Here, we present the structure of an outer-membrane core complex from the iconic F-T4SS encoded by the E. coli pED208 plasmid solved by single-particle cryo-electron microscopy at 3.3 Å resolution. This 2.1 MDa structure, provides an atomic model of the TraB, TraK and TraV proteins and unveils unique stoichiometry relationships between the three proteins. Surprisingly, the complex is formed by two highly flexible concentric rings made by a total of 69 proteins chains arranged in two distinct symmetries. The components that make up this complex include the proteins TraB, TraK and TraV which are homologous to VirB10, VirB9 and VirB7 respectively and are observed throughout the multi-functional T4SS spectrum.

In the inner ring, seventeen ASUIR heterodimers made of TraBCTD and TraVNTD (labelled −8 to +8 in the clockwise direction) assemble to form the complete OMCCIR. In the ASUIR, an atomic model of the TraB C-terminal domain (CTD) and TraV N-terminal domain (NTD) could be built and refined into the electron density. The ASUIR is predominantly made up of TraBCTD which includes a total of seventeen β strands and three α helices. Six of these strands (β3, β5, β8, β14–β16) mediate the interaction with TraVNTD. The core of the structure has a β barrel that connects to two anti-parallel α helices (α1 and α2) and a third helix (α3) towards the C-terminal end. The N-terminal end of the TraV (residues 17–54) is located entirely in the inner ring which includes a single helix α1. A single ASUIR makes contact with four other neighbouring ASUs, involving two ASUs each in the clockwise and anti-clockwise direction. The ASUs +1 and −1 are contiguous to ASU-0IR and hence bury a much larger surface area of 2481 Å2 and 2435 Å2, respectively. Notably, an inter TraVNTD di-sulphide bond has been observed between residue Cys35 of chain B and Cys27 of chain D. This interchain di-sulphide bond between contiguous TraVNTD chains creates a wide mesh that spreads over the TraB proteins and extends to the periphery of the OMCCIR. The TraB α1 helix and TraV NTD residues Gly17-Ser23 define a rim-ward hydrophobic surface suggesting that this portion of the OMCC is likely embedded in the bacterial OM.

>MANVNKVVRRRQVALLIALVLGIGAGGAGTWMVSEMNLKKAPPAKAPKGEPAPDMTGVVNQSFDNKVQRSAIAEAQRLNKETQTEIKKLRTEMGLVSRDLKGSQDRIRELEDQNQLLQTQLEAGKNFDSLSAEPLPGALASQGKPAPAGNVPPPTSFWPAGGGQAPAAPVMTPIQRPGMMDSQEFSLPDTGPKKPRFPWISSGSFVEAIVVEGADANASVTGDKNTAPMQLRLTGKVQMPNDEEFDLTGCFVTLEAWGDVSSERAIVRSRSISCKLGDDDIDQKIAGHVSFMGKNGIKGEVVMRNGQILLYAGGAGFLDGIGKGIEKASSTTVGVGATASMSAADIGQAGLGGGVSSAAKTLSDYYIKRAEQYHPVIPIGAGNEVTLVFQDGFQLETLEEARAKAAARKKQNQPSASSTPAAMPGNTPDMLKQLQDFRVGDTVDPATGQVVTQWSHPQFEK[17x];>[17x]MKKITLLLAGSALLLSGCAGVKSSFDCDATTSDTCMTMTKANQLARDKAAKQAGKPAAGGLPSLVNLPATSAVEVPSASRSAVTPPSGTRTVSTTPPVSAGTSAGVNTNTTTSTLTPRPVAGTPVTTTPSSVAYRPVVSVVTPTPSCQNVRCDNPGTVHPQRSRDQIATVWIAPWVDSDNAFHQPGRVSFVVSPADWVLPARVN> PKPGDIFEVELAKNDNSLGISVTGGVNTSVRHGGIYVKAVIPQGAAESDGRIHKGDRVLAVNGVSLEGATHKQAVETLRNTGQVVHLLLE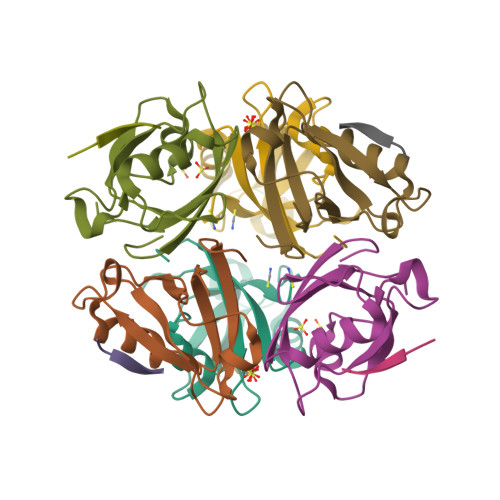KGQSPT;> EQVSAV> MAYIKRVIIKGFKTYRNETIIDNFSPHQNVIIGSNGSGKSNFFAAIRFVLSDDYSNLKREERQGLIHQGSGGSVMSASVEIVFHDPDHSMILPSGVLSRGDDEVTIRRTVGLKKDDYQLNDRNVTKGDIVRMLETAGFSMNNPYNIVPQGKIVALTNAKDKERLQLLEDVVGAKSFEVKLKASLKKMEETEQKKIQINKEMGELNSKLSEMEQERKELEKYNELERNRKIYQFTLYDRELNEVINQMERLDGDYNNTVYSSESSKHPTSLVPRGSDITSDQLLQRLNDMNTEISGLKNVNKRAFENFKKFNERRKDLAERASELDESKDSIQDLIVKLKQQKVNAVDSTFQKVS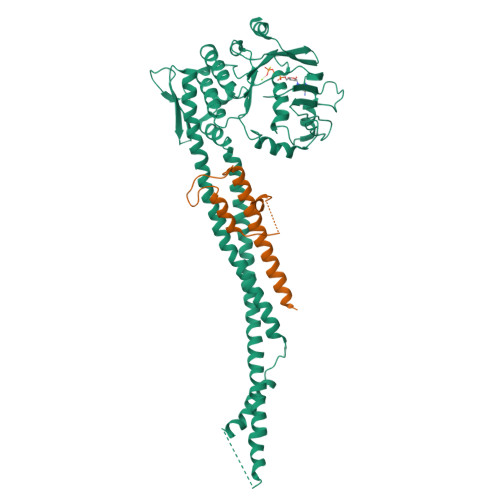ENFEAVFERLVPRGTAKLIIHRKNDNANDHDESIDVDMDAESNESQNGKDSEIMYTGVSISVSFNSKQNEQLHVEQLSGGQKTVCAIALILAIQMVDPASFYLFDEIDAALDKQYRTAVATLLKELSKNAQFICTTFRTDMLQVADKFFRVKYENKISTVIEVNREEAIGFIRGSNKFAEVWSHPQFEK;> MVTENPQRLTVLRLATNKGPLAQIWLASNMSNIPRGSVIQTHIAESAKEIAKASGCDDESGDNEYITLRTSGELLQGIVRVYSKQATFLLTDIKDTLTKISMLFKTSQKMTSTVNHHHHHH> MAGKKGQKKSGLGNHGKNSDMDVEDRLQAVVLTDSYETRFMPLTAVKPRCLLPLANVPLIEYTLEFLAKAGVHEVFLICSSHANQINDYIENSKWNLPWSPFKITTIMSPEARCTGDVMRDLDNRGIITGDFILVSGDVLTNIDFSKMLEFHKKMHLQDKDHISTMCLSKASTYPKTRTIEPAAFVLDKSTSRCIYYQDLPLPSSREKTSIQIDPELLDNVDEFVIRNDLIDCRIDICTSHVPLIFQENFDYQSLRTDFVKGVISSDILGKHIYAYLTDEYAVRVESWQTYDTISQDFLGRWCYPLVLDSNIQDDQTYSYESRHIYKEKDVVLAQSCKIGKCTAIGSGTKIGEGTKIENSVIGRNCQIGENIRIKNSFIWDDCIIGNNSIIDHSLIASNATLGSNVRLNDGCIIGFNVKIDDNMDLDRNTKISASPLKNAGSRMYDNESNEQFDQDLDDQTLAVSIVGDKGVGYIYESEVSDDE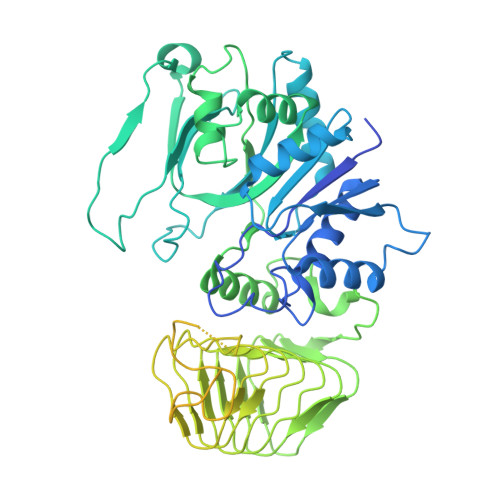DSSTEACKEINTLSNQLDELYLSDDSISSATKKTKKRRTMSVNSIYTDREEIDSEFEDEDFEKEGIATVERAMENNHDLDTALLELNTLRMSMNVTYHEVRIATITALLRRVYHFIATQTLGPKDAVVKVFNQWGLLFKRQAFDEEEYIDLMNIIMEKIVEQSFDKPDLILFSALVSLYDNDIIEEDVIYKWWDNVSTDPRYDEVKKLTVKWVEWLQNADEESSSEEE PHENYLALANINE AMIDE | C9 H12 N2 O | 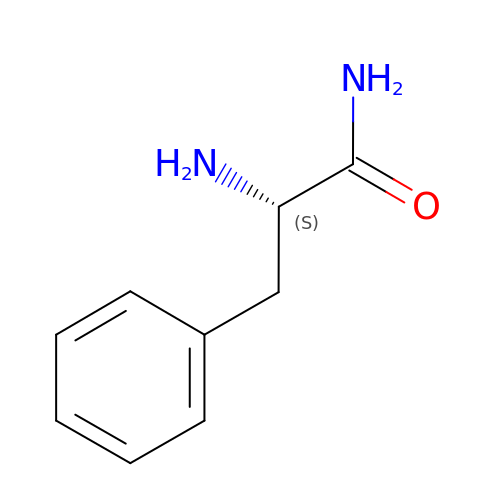OBSIQMZKFXFYLV-QMMMGPOBSA-N> GPGSEFSLDHSDLVAELLKELSNHNERVEERKIALYELMKLTQEESFSVWDEHFKTILLLLLETLGDKEPTIRALALKVLREILRHQPARFKNYAELTVMKTLEAHKDPHKEVVRSAEEAASVLATSISPEQCIKVLCPIIQTADYPINLAAIKMQTKVIERVSKETLNLLLPEIMPGLI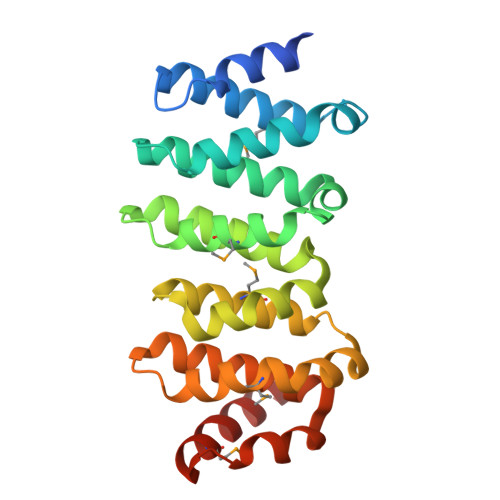QGYDNSESSVRKACVFCLVAVHAVIGDELKPHLSQLTGSKMKLLNLYIKRAQTGS> MTTELNQGEQFVADFRANAAALTTANAYNPEDEHDACGVGFIAAIDGKPRRSVVEKGIEALKAVWHRGAVDADGKTGDGAGIHVAVPQKFFKDHVKVIGHRAPDNKLAVGQVFLPRISLDAQEACRCIVETEILAFGYYIYGWRQVPINVDIIGEKANATRPEIEQIIVGNNKGVSDEQFELDLYIIRRRIEKAVKGEQINDFYICSLSARSIIYKGMFLAEQLTTFYPDLLDERFESDFAIYHQRYSTNTFPTWPLAQPFRMLAHNGEINTVKGNVNWMKAHETRMEHPAFGTHMQDLKPVIGVGLSDSGSLDTVFEVMVRAGRTAPMVKMMLVPQALTSSQTTPDNHKALIQYCNSVMEPWDGPAALAMTDGRWVVGGMDRNGLRPMRYTITTDGLIIGGSETGMVKIDETQVIEKGRLGPGEMIAVDLQSGKLYRDRELKDHLATLKPWDKWVQNTTHLDELVKTASLKGEPSDMDKAELRRRQQAFGLTMEDMELILHPMVEDGKEAIGSMGDDSPIAVLSDKYRGLHHFFRQNFSQVTNPPIDSLRERRVMSLKTRLGNLGNILDEDETQTRLLQLESPVLTTAEFRAMRDYMGDTAAEIDATFPVDGGPEALRDALRRIRQETEDAVRGGATHVILTDEAMGPARAAIPAILATGAVHTHLIRSNLRTFTSLNVRTAEGLDTHYFAVLIGVGATTVNAYLAQEAIAERHRRGLFGSMPLEKGMANYKKAIDDGLLKIMSKMGISVISSYRGGGNFEAIGLSRALVAEHFPAMVSRISGIGLNGIQKKVLEQHATAYNEEVVALPVGGFYRFRKSGDRHGWEGGVIHTLQQAVTNDSYTTFKKYSEQVNKRPPMQLRDLLELRSTKAPVPVDEVESITAIRKRFITPGMSMGALSPEAHGTLNVAMNRIGAKSDSGEGGEDPARFRPDKNGDNWNSAIKQVASGRFGVTAEYLNQCRELEIKVAQGAKPGEGGQLPGFKVTEMIARLRHSTPGVMLISPPPHHDIYSIEDLAQLIYDLKQINPDAKVTVKLVSRSGIGTIAAGVAKANADIILISGNSGGTGASPQTSIKFAGLPWEMGLSEVHQVLTLNRLRHRVRLRTDGGLKTGRDIVIAAMLGAEEFGIGTASLIAMGCIMVRQCHSNTCPVG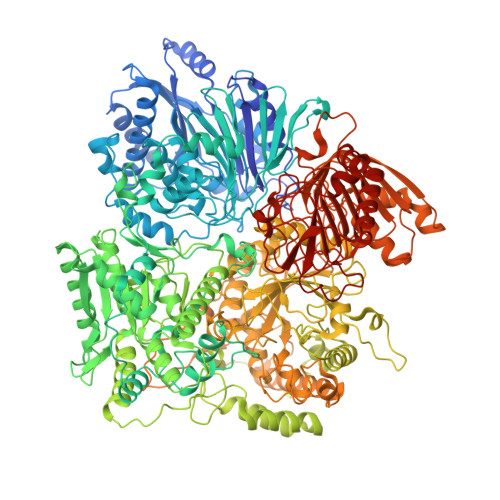VCVQDDKLRQKFVGTPEKVVNLFTFLAEEVREILAGLGFRSLNEVIGRTDLLHQVSRGAEHLDDLDLNPRLAQVDPGENARYCTLQGRNEVPDTLDARIVADARPLFEEGEKMQLAYNARNTQRAIGTRLSSMVTRKFGMFGLQPGHITIRLRGTAGQSLGAFAVQGIKLEVMGDANDYVGKGLSGGTIVVRPTTSSPLETNKNTIIGNTVLYGATAGKLFAAGQAGERFAVRNSGATVVVEGCGSNGCEYMTGGTAVILGRVGDNFAAGMTGGMAYVYDLDDSLPLYINDESVIFQRIEVGHYESQLKHLIEEHVTETQSRFAAEILNDWAREVTKFWQVVPKEMLNRLEVPVHLPKAISAE> ARTKQ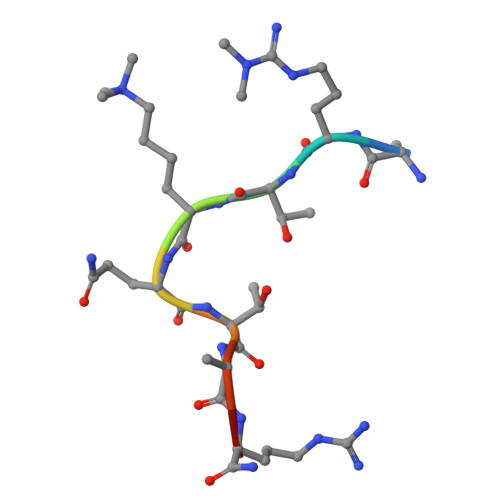TARA>MKEFYISIETVGNNIVERYIDENGKERTREVEYLPTMFRHCKEESKYKDIYGKNCAPQKFPSMKDARDWMKRMEDIGLEALGMNDFKLAYISDTYGSEIVYDRKFVRVANCDIEVTGDKFPDPMKAEYEIDAITHYDSIDDRFYVFDLLNSMYGSVSKWDAKLAAKLDCEGGDEVPQEILDRVIYMPFDNERDMLMEYINLWEQKRPAIFTGWNIEGFAVPYIMNRVKMILGERSMKRFSPIGR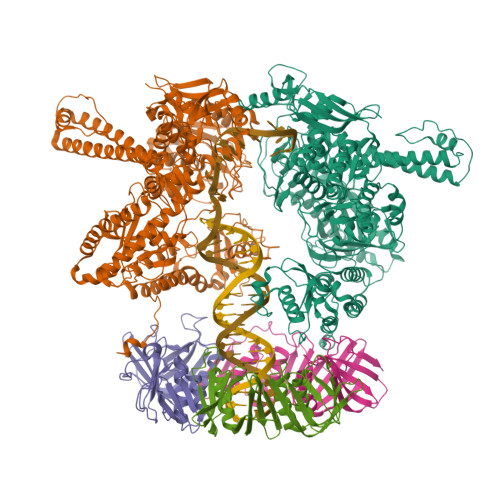VKSKLIQNMYGSKEIYSIDGVSILDYLDLYKKFAFTNLPSFSLESVAQHETKKGKLPYDGPINKLRETNHQRYISYNIIDVESVQAIDKIRGFIDLVLSMSYYAKMPFSGVMSPIKTWDAIIFNSLKGEHKVIPQQGSHVKQSFPGAFVFEPKPIARRYIMSFDLTSLYPSIIRQVNISPETIRGQFKVHPIHEYIAGTAPKPSDEYSCSPNGWMYDKHQEGIIPKEIAKVFFQRKDWKKKMFAEEMNAEAIKKIIMKGAGSCSTKPEVERYVKFSDDFLNELSNYTESVLNSLIEECEKAATLANTNQLNRKILINSLYGALGNIHFRYYDLRNATAITIFGQVGIQWIARKINEYLNKVCGTNDEDFIAAGDTDSVYVCVDKVIEKVGLDRFKEQNDLVEFMNQFGKKKMEPMIDVAYRELCDYMNNREHLMHMDREAISCPPLGSKGVGGFWKAKKRYALNVYDMEDKRFAEPHLKIMGMETQQSSTPKAVQEALEESIRRILQEGEESVQEYYKNFEKEYRQLDYKVIAEVKTANDIAKYDDKGWPGFKCPFHIRGVLTYRRAVSGLGVAPILDGNKVMVLPLREGNPFGDKCIAWPSGTELPKEIRSDVLSWIDHSTLFQKSFVKPLAGMCESAGMDYEEKASLDFLFG[2x];>[3x]MKLSKDTTALLKNFATINSGIMLKSGQFIMTRAVNGTTYAEANISDVIDFDVAIYDLNGFLGILSLVNDDAEISQSEDGNIKIADARSTIFWPAADPSTVVAPNKPIPFPVASAVTEIKAEDLQQLLRVSRGLQIDTIAITVKEGKIVINGFNKVEDSALTRVKYSLTLGDYDGENTFNFIINMANMKMQPGNYKLLLWAKGKQGAAKFEGEHANYVVALEADSTHDF>MKKRLLLPLFAALCLSQIAHADEGMWLMQQLGRKYAQMKERGLKMKEYDLYNPNGTSLKDAVVLFDGGCTGEVVSDRGLVLTNHHCGYDMIQAHSTLEHNYLENGFWAMREADELPNKDISVVFIDKIEDVTDYVKKELKAIKDPNSMDYLSPKYLQKLADKKAGKNFSAKNPGLSVEIKAFYGGNLYLMFTKKTYTDVRLVGAPPSSIGKFGADTDNWIWPRHTGDFSIFRIYADKNGNPAPYSE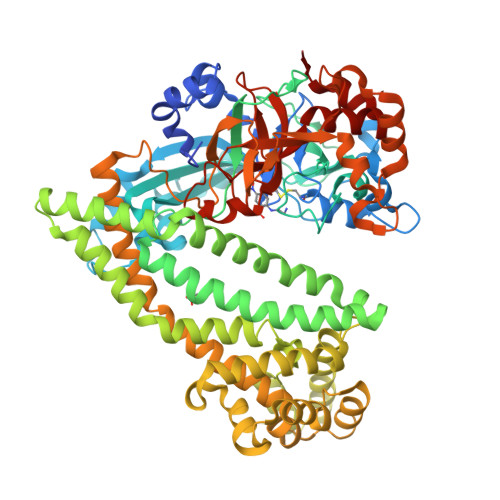DNVPLKPKRFFNISLGGVQENDYAMIMGFPGTTHRYFTASEVDEWKSIDNDIRIRMRDIRQGVMLREMLADPQIKIMYSAKYAASQNAYKRAIGANWAIKTRGLRQNKQAMQDRLIAWGAKQGTPRYEEAVHEIDATVAKRADLRRRYWMIEEGIIRGIEFARSPIPTEDETKALQGNDASARKEAIDKIRTRYSKFANKDYSAEVDKKVAVAMLTEYLKEIPYENLPLHLRLVKDRFAGDVQAYVDDIFARSVFGSEAQFDAFAAVPSVEKLAEDPMVLFASSVFDEYRKLYNELRPYDDPILRAQRTYIAGLLEMDGDQDQFPDANLTLRFTYGQVKGYSPRDNVYYGHQTTLDGVMEKEDPDNWEFVVDPKLKAVYERKDFGRYADRSGRMPVAFCATTHTTGGNSGSPVMNANGELIGLNFDRNWEGVGGDIQYLADYQRSIIVDIRYVLLVIDKVGGCQRLLDEMNIVP[2x]>[8x]DDVTVVYQNGLPVISVRLPSRRERCQFTLKPISDSVGVFLRQLQEEDRGIDRVAIYSPDGVRVAASTGIDLLLLDDFKLVINDLTYHVRPPKRDLLSHENAATLNDVKTLVQQLYTTLCIEQHQLNKERELIERLEDLKEQLAPLEKVRIEISRKAEKRTTLVLWGGLAYMATQFGILARLTWWEYSWDIMEPVTYFITYGSAMAMYAYFVMTRQEYVYPEARDRQYLLFFHKGAKKSRFDLEKYNQLKDAIAQAEMDLKRLRDPLQVHLPLRQIG;>[8x]VIVTRSGAILPKPVKMSFGLLRVFSIVIPFLYVGTLISKNFAALLEEHDIFVPE

The Ca2+ influx is mediated by MCU, driven by membrane potential and using a uniporter mechanism. Patch-clamp analysis of MCU currents demonstrated that MCU is a channel with exceptionally high Ca2+ selectivity. The MCU subunit comprises three structural domains: the transmembrane domain (TMD), the coiled-coil domain (CCD), and the N-terminal domain (NTD). The TMD of MCU is known to be responsible for Ca2+ selectivity and conduction, and each MCU subunit contributes two transmembrane helices to the TMD: TM1 and TM2.

The NTD is connected to the CC1 via the linking helix α1, and the four α1 helices of each MCU subunits stably interact with each other, forming a four-helix bundle that stabilizes the MCU tetramers. In our structure, four EMREs, four CDLs, four horizontal PCs, and four vertical PCs form a cage and bundle up the four MCU subunits. The N-terminal (48–65) and C-terminal (97–107) residues of EMRE appear as loops, while its middle residues (66–96) adopt the configuration of a single α-helix. This α-helix locates within the membrane and is tilted by 37° relative to the normal vector of membrane, such that each EMRE subunit interacts with two neighboring MCU subunits. In the MEMMS structure, one CDL and one horizontal PC molecules insert into the gap between TM1 and TM2 of each MCU subunit, and another vertical PC molecule stands alongside each TM2. Notably, most of the lipid chains of the CDL and vertical PC in our structure are parallel to the helices of TMD, while the lipid chains of the horizontal PC are positioned horizontally in the membrane. In addition to interacting with TM1, TM2, and CC2 of one MCU subunit, each CDL molecule also interacts tightly with the neighboring EMRE. Specifically, a highly conserved residue of MCU CC2, R297, can form salt bridge with the phosphate group of CDL and hydrogen bonds with the main chain oxygen of V61 in EMRE. We mutated R297 to aspartate, and strikingly this mutation completely abolished the Ca2+ uptake via MCU. Similarly, P60A mutation in EMRE, just next to the MCU-R297, can also totally abolish MCU activity, proving that the correct interactions between CC2 and EMRE are important to MEMMS.> MPRWY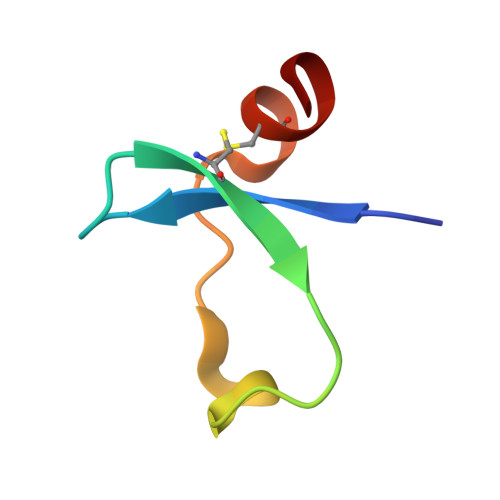FDLSKGKCVRFIYGGCGGNRNNFESEDYCMAVC>GPGTSRQCQEQLKEVNKTCEALLFKLGEKVKTLEMEVAKEKAVCSKDKESLLAGKRQTEEQLEA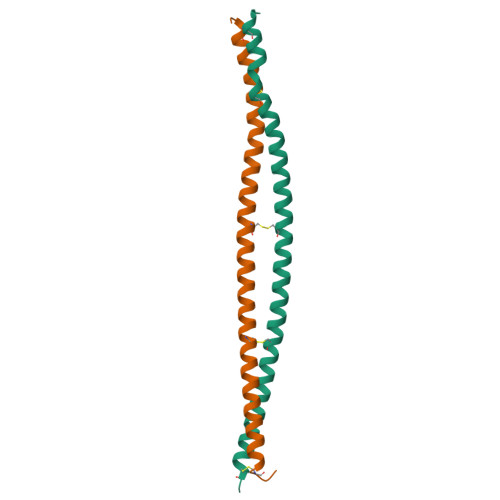CGKARERQQQEQQVTEENLRKVQSLCIPLDQ[4x]5-(6,7-dihydro-4~{H}-thieno[3,2-c]pyridin-5-ylcarbonyl)-1-methyl-pyridin-2-one 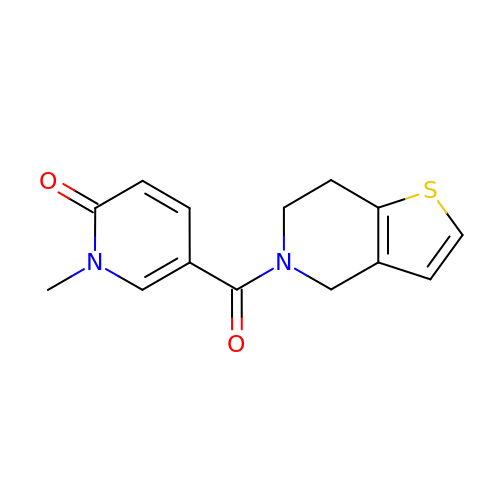| C14 H14 N2 O2 S | PXCRFQLKGNEWBG-UHFFFAOYSA-N>MTKLILIRHGETEWNLLGKIQGCTDIELTPNGIQQANEVAQQIKGNFDIIYSSPLHRALITAQKIAGDKEVHLIEGMKEIPFGTWEGHTFEELNGDINYKKFLSGEDGCPFDSTGMSIASWSKKNAQLLLDLCKQNENKTI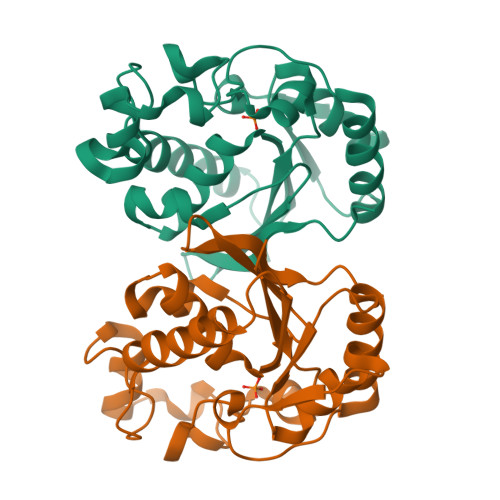VCVSHGAWIKTSILGLLEMEPTMYHKFQLGNTGITTFIFRHGHPVLTSFNSTQHLLTENKSKTGHHHHHH[4x]> MMRSSSFCRRQIRPYYNLPSKSEHGRKMTGFLTPYRHWMWKQNELWRNVHEAQFEHLRRV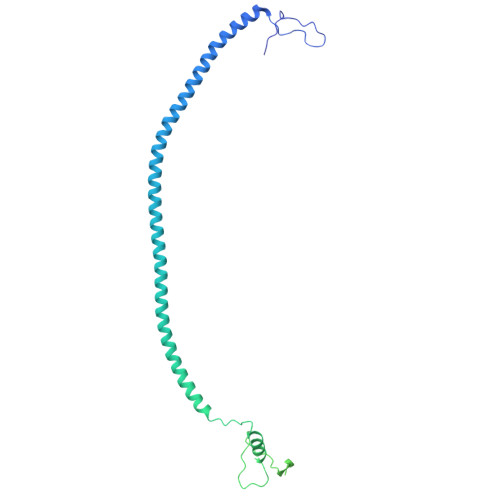YKRQWLESFRVNADEYIYKYNITKAAQLAQWECEMKEQEKKRIEARQMMDGRQALKKKHLDLLREFHERQFFFWYERASERLQNMNLINYVPHAQLREHIDKELDKYVAGKNEPYPLNFVGQMPFLEDGDGNIVEVPESLLSNHMAEHPDSTAKPHEPHTSSSISEAAAFEERMLRAMVSAKEEDLKEWLGDDSRALSETIDDISREEEEREADIRVARSMEETDAEREVSRRAYIERGKTGSRSIFRPPTVSEGAGGTPSAPAGDANTPMRRRKKGKLDRVHALQAHQDELLAKLSSQGLKEGVDASSVPERGKIVQSRGRIRDKAVIPTHEVLMQKPELAAGSTPGARIQTKDMVDKMYHRGKYKKSGSGDKSDGEDL>[11x]RIKTNAAVAAVLPANEDQADYPSTFFEGGNEIRLYVNRGEKLDVLRQYVYMGLVEKNCRIQHVNAYLYAVLKGERELLEADWDSFGHKIGIQGDKIGPFNLVRVEDIPDGLPDGKLNAEVSAE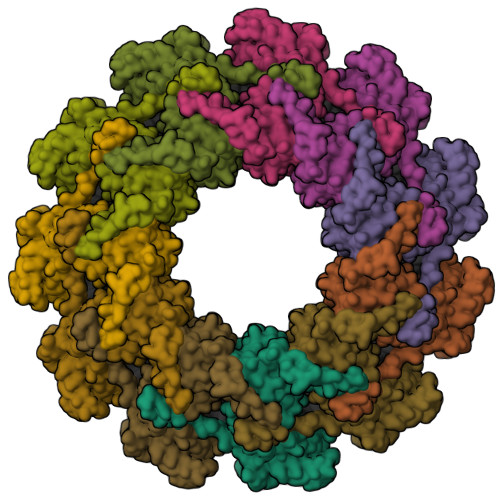DDAWLPLFLLGLYRVGRASETAYRTLLMESLIKQCKAIKSDWVSPVTATHKYFDVWGNDGNYLKIVACVDMFYNHFKKSIKATFRWGTIVSRFKDCAALATLGHVVKITGLTIEEVFTWVLQTEVADELVKMMKPGQEIDKSTSYMPYLIDMGISAKSPYSTIKNPSFHFWGQLVAALCRSKRALNARQPDEIDSMSISNASLLMAYALGSSPDIEQQFSTGNTYRKPPKEASYLVSEEPKNRSVVEWIAWYSDVDNKPTDDMLMMAKRVAGTISGPRDNSVGKWIKQTYG O-[(2R,3S,4R,5R)-5-(4-amino-2-oxopyrimidin-1(2H)-yl)-4-hydroxy-2-(hydroxymethyl)tetrahydrofuran-3-yl] O-{[(2R,3S,4R,5R)-5-(2,4-dioxo-3,4-dihydropyrimidin-1(2H)-yl)-3,4-dihydroxytetrahydrofuran-2-yl]methyl} hydrogen (S)-phosphorothioate 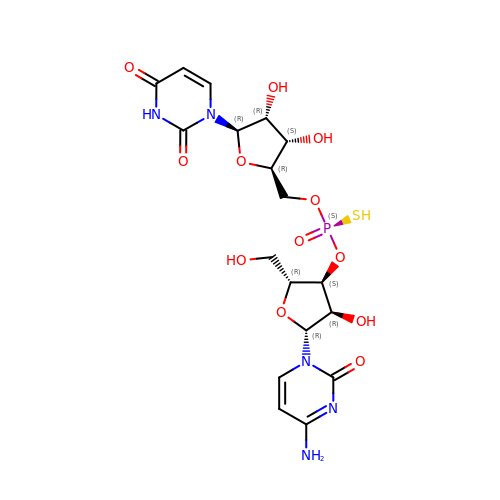| C18 H24 N5 O12 P S | VZQLNJPTHATNOF-OXIRAOGTSA-N> GLIVDTRDVEERVHVMRKTALAPTVAHGVFNPEFGPAALSNKDPRLNEGVVLDEVIFSKHKGDTKMSAEDKALFRRCAADYASRLHSVLGTANAPLSIYEAIKGVDGLDAMEPDTAPGLPWALQGKRRGALIDFENGTVGPEVEAALKLMEKREYKFACQTFLKDEIRPMEKVRAGKTRIVDVLPVEHILYTRMMIGRFCAQMHSNNGPQIGSAVGCNPDVDWQRFGTHFAQYRNVWDVDYSAFDANHCSDAMNIMFEEVFRTEFGFHPNAEWILKTLVNTEHAYENKRITVEGGMPSGCSATSIINTILNNIYVLYALRRHYEGVELDTYTMISYGDDIVVASDYDLDFEALKPHFK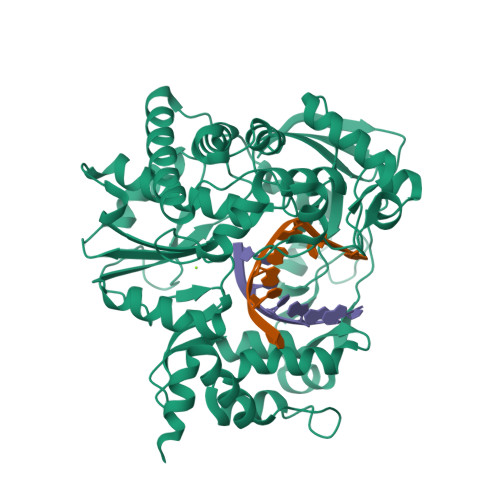SLGQTITPADKSDKGFVLGHSITDVTFLKRHFHMDYGTGFYKPVMASKTLEAILSFARRGTIQEKLISVAGLAVHSGPDEYRRLFEPFQGLFEIPSYRSLYLRWVNAVCGDAAAALEHHHHHH> GSAMAKANSSFSEVQIARR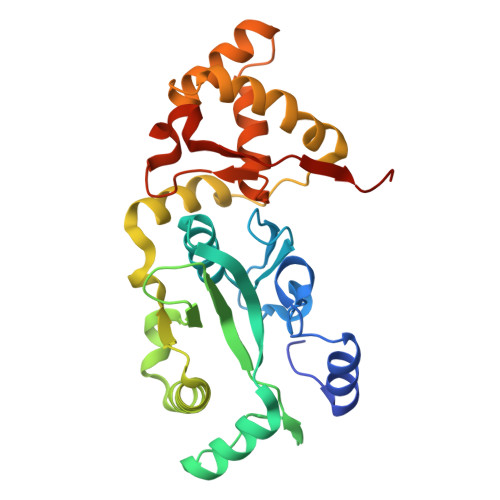IKEGRGQGHGKDYIPWLTVQEVPSSGRSHRIYSHKTGRVHHLLSDLELAVFLSLEWESSVLDIREQFPLLPSDTRQIAIDSGIKHPVIRGVDQVMSTDFLVDCKDGPFEQFAIQVKPAAALQDERTLEKLELERRYWQQKQIPWFIFTDKEINPVVKENIEWLYSVKTEEVSAELLAQLSPLAHILQEKGDENIINVCKQVDIAYDLELGKTLSEIRALTANGFIKFNIYKSFRANKCADLCISQVVNMEELRYVAN>MVLYFIGLGLYDERDITVKGHEIAKKCDYVFAEFYTSLMAGTTLGRIQKLIGKEIRVLSREDVELNFENIVLPLAKENDVAFLTPGDPLVATTHAELRIRAKRAGVESYVIHAPSIYSAVGITGLHIYKFGKSATVAYPEGNWFPTSYYDVIKENAERGLHTLLFLDIKAEKRMYMTANEAMELLLKVEDMKKGGV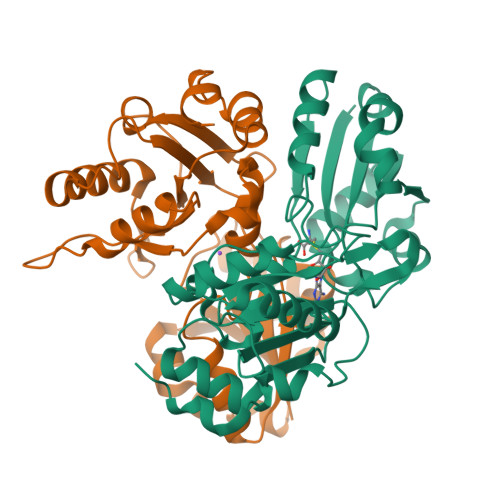FTDDTLVVVLARAGSLNPTIRAGYVKDLIREDFGDPPHILIVPGKLHIVEAEYLVEIAGAPREILRVNV[2x]>MIELVIVSRLLEYPDAALWQHQQEMFEAIAASKNLPKEDAHA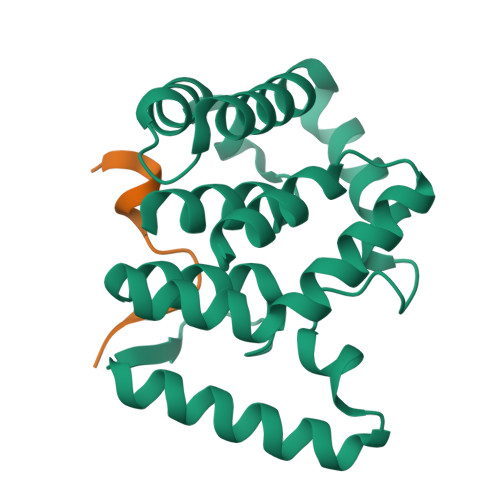LGIFLRDLTTMDPLDAQAQYSELFDRGRATSLLLFEHVHGESRDRGQAMVDLLAQYEQHGLQLNSRELPDHLPLYLEYLAQLPQSEAVEGLKDIAPILALLSARLQQRESRYAVLFDLLLKLANTAIDSDKVAEKIADEARPGAHHHHHH[2x];>[2x]MSKFLDRFRYFKQKG>[2x]GAMGCSWIEMDGKVHKFTA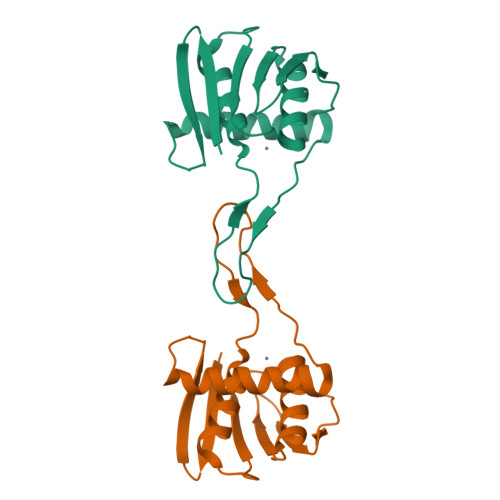RDKSHPESKEIYEKLSEVTRKLEREVGYVADTKFVLHNVDEGEKVQMLHGHSERIAIAYGLLRTPDRACLRITKNLRVCRDCHTFCKLVSKLFRRDIVMRDANRFHHFESGLCSCGDSW> MVGSLNCIVAVSQNMGIGKNGDLPWPPLRNEFRYFKRMTTTSSVEGKQNLVIMGKKTWFSIPEKNR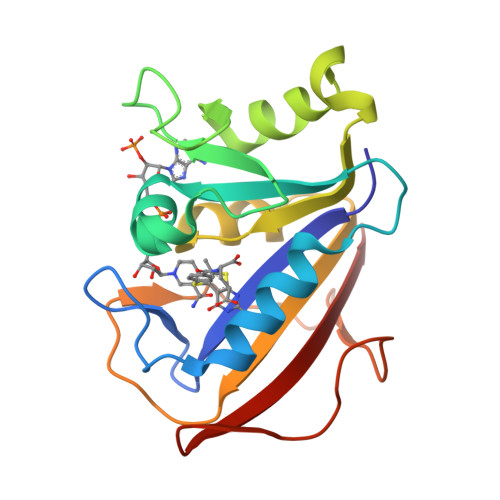PLKGRINLVLSRELKEPPQGAHFLSRSLDDALKLTEQPELANKVDMVWIVGGSSVYKEAMNHPGHLKLFVTRIMQDFESDTFFPEIDLEKYKLLPEYPGVLSDVQEEKGIKYKFEVYEKND> MLPPGKPEIFKCRSPNKETFTCWWRPGTDGGLPTNYSLTYHREGETLMHECP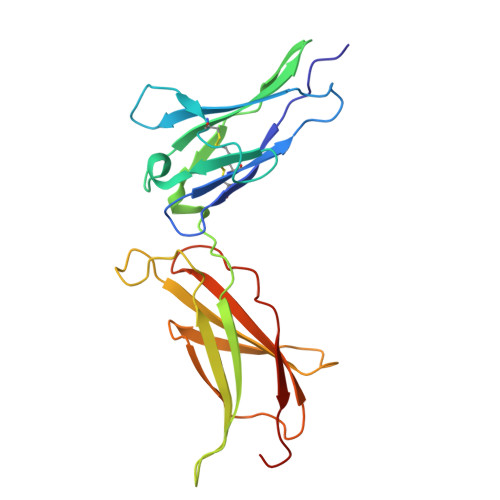DYITGGPNSCHFGKQYTSMWRTYIMMVNATNQMGSSFSDELYVDVTYIVQPDPPLELAVEVKQPEDRKPYLWIKWSPPTLIDLKTGWFTLLYEIRLKPEKAAEWEIHFAGQQTEFKILSLHPGQKYLVQVRCKPDHGYWSAWSPATFIQIPSDFTMND>[4x]MEPSALRKAGSEQEEGFEGLPRRVTDLGMVSNLRRSNSSLFKSWRLQCPFGNNDKQESLSSWIPENIKKKECVYFVESSKLSDAGKVVCQCGYTHEQHLEEATKPHTFQGTQWDPKKHVQEMPTDAFGDIVFTGLSQKVKKYVRVSQDTPSSVIYHLMTQHWGLDVPNLLISVTGGAKNFNMKPRLKSIFRRGLVKVAQTTGAWIITGGSHTGVMKQVGEAVRDFSLSSSYKEGELITIGVATWGTVHRREGLIHPTGSFPAEYILDEDGQGNLTCLDSNHSHFILVDDGTHGQYGVEIPLRTRLEKFISEQTKERGGVAIKIPIVCVVLEGGPGTLHTIDNATTNGTPCVVVEGSGRVADVIAQVANIPVSDITISLIQQKLSVFFQEMFETFTESRIVEWTKKIQDIVRRRQLLTVFREGKDGQQDVDVAILQALLKASRSQDHFGHENWDHQLKLAVAWNRVDIARSEIFMDEWQWKPSDLHPTMTAALISNKPEFVKLFLENGVQLKEFVTWDTLLYLYENLDPSCLFHSKLQKVLVEDPERPACAPAAPRLQMHHVAQVLRELLGDFTQPLYPRPRHNDRLRLLLPVPHVKLNVQGVSLRSLYKRSSGHVTFTMDPIRDLLIWAIVQNRRELAGIIWAQSQDCIAAALACSKILKELSKEEEDTDSSEEMLALAEEYEHRAIGVFTECYRKDEERAQKLLTRVSEAWGKTTCLQLALEAKDMKFVSHGGIQAFLTKVWWGQLSVDNGLWRVTLCMLAFPLLLTGLISFREKRLQDVGTPAARARAFFTAPVVVFHLNILSYFAFLCLFAYVLMVDFQPVPSWCECAIYLWLFSLVCEEMRQLFYDPD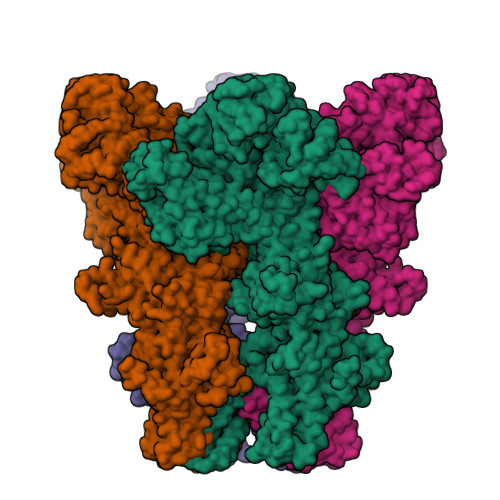ECGLMKKAALYFSDFWNKLDVGAILLFVAGLTCRLIPATLYPGRVILSLDFILFCLRLMHIFTISKTLGPKIIIVKRMMKDVFFFLFLLAVWVVSFGVAKQAILIHNERRVDWLFRGAVYHSYLTIFGQIPGYIDGVNFNPEHCSPNGTDPYKPKCPESDATQQRPAFPEWLTVLLLCLYLLFTNILLLNLLIAMFNYTFQQVQEHTDQIWKFQRHDLIEEYHGRPAAPPPFILLSHLQLFIKRVVLKTPAKRHKQLKNKLEKNEEAALLSWEIYLKENYLQNRQFQQKQRPEQKIEDISNKVDAMVDLLDLDPLKRSGSMEQRLASLEEQVAQTAQALHWIVRTLRASGFSSEADVPTLASQKAAEEPDAEPGGRKKTEEPGDSYHVNARHLLYPNCPVTRFPVPNEKVPWETEFLIYDPPFYTAERKDAAAMDPMGDTLEPLSTIQYNVVDGLRDRRSFHGPYTVQAGLPLNPMGRTGLRGRGSLSCFGPNHTLYPMVTRWRRNEDGAICRKSIKKMLEVLVVKLPLSEHWALPGGSREPGEMLPRKLKRILRQEHWPSFENLLKCGMEVYKGYMDDPRNTDNAWIETVAVSVHFQDQNDVELNRLNSNLHACDSGASIRWQVVDRRIPLYANHKTLLQKAAAEFGAHY Viral transcription is highly regulated, as demonstrated biochemically in viruses of the Reoviridae. mRNA transcription in these viruses is activated by external actions, for example, removal of their outer shell in multi-shelled reoviruses and binding of S-adenosyl-L-methionine (SAM) in the single-shelled cytoplasmic polyhedrosis virus (CPV). To reveal the mechanisms of transcriptional regulation of viruses within the Reoviridae family, we determined the cryoEM structures of six CPV/ligand complexes in the presence of magnesium ion: CPV+SAM (i.e., ‘S-CPV’), CPV+SAM+4 nucleoside triphosphates (NTPs) (i.e., transcribing, or ‘t-CPV’), CPV+SAM+GTP+ATP (i.e., ‘SGA-CPV’), CPV+SAM +GTP (i.e., ‘SG-CPV’), CPV+GTP (i.e., ‘G-CPV’), and CPV+ATP (i.e., ‘A-CPV’) at resolutions ranging from 2.9 to 3.1 Å. Like the atomic model of unliganded CPV, the atomic models of these liganded CPV all contain two conformers of the capsid shell proteins (CSP-A and CSP-B), two conformers of the large protrusion proteins (LPP-3 and LPP-5), and one conformer of TP in each asymmetrical unit. We discovered that the large sub-domain of guanylyltransferase (GTase) domain of CPV turret protein (TP) also has an ATP-binding site and is likely an ATPase that mediates the activation process of viral RNA transcription and capping.

Except for A-CPV, these atomic models also contain ligands revealed in our cryoEM maps. To test this hypothesis, we first obtained the 3D reconstructions of G-CPV and A-CPV at 2.9 Å and 3.1 Å resolutions, respectively. Our structures of G-CPV and A-CPV show that, in the absence of SAM, neither GTP nor ATP induced any conformational change.

> MWHYTSINNDTRVALDPKPNQIRTITKPNTVPQLGTDYLYTFNSQRRSHTLRLLGPFQYFNFSETDRGHPLFRLPLKYPSKAIPADELIDNLHSWMRSVHLLHVRSEDNTLRYNWMLGVYARSTNYTTPVGQLVVNAPAILNYSNPQDAFNSVFVALGIDYIDIPITNSNIFDDSSTPYNVRIWHAPTMTEVNHILALMRKSTLVSTHSSWHWNVLHTFHYRSESDMIDHFAAKILEDWRQKEKLDKGALVEADRVIQRLIPLSSSTYVQRLAAIGALYPNEFTENVLDLSRLSTALLQLSDTYYQHANDQLRRLYRRMYNDSRTLYMTQRHQELLLAQITADPNILLYPYTYIFTTIPTSMNYISNTGQGRIKHSLTVTGATEHDTVADIVLGQTGEDVITISMVEPMSIAVEDMYGYVLDTPTRDIWPADEQIEQKGDAVALYDTKTSRALGMFNNTVRIDDLLSPLLSLVYRTYIKGDTMTMTQGSLDHLTLCAAVDSDITFVGNRMIAPLPEGYIPKPMHRNNSTMKMLSLYVALKKLENFATNSYLMAPDTSIILLGAEREPAVNILRRFNRNVSNVRIIGMGDRAVEPNIRVRVPFPIDKNISADFIICDINSYEDQSFESMFSETISVVTTCASAATRALVKINHPSEYMINSVIERLSQLGGVFYHTALLKTASQNPYSYETYIYITPIAAAVRFPFYSNSAMINRYMTAVADDEMPIIPSIHTVIKGHSNTYSPGLFCGCVDVQSAPLALSQLKSYCSEATTWRVDSDDNLVNIIARIDPARIALEFRTRSNTSAYHEYQRYVPNGLGFKVRKTREFRYMHREVTFIHKLMMYALIREQISLTENMTQVVSIGGRNLADISVVPLNMKYVVIDPATRIETLTQEKKNIEVQSRPFQFDAANMDLENNSIYLFIAVIMNEPNGAATPARMQMDKIRNVATAMLTRTNCVAYISFYEAGIITRLDQSTAHKTIRVEEGRLKVANYVPVDTLVEADVTLMLRDIGITHEIIRPSTPELIDACSNYGIRLGSTGGAVLDVFNHYSPVIKLVRS;>MHSTNNNSNKRNNEEKHKQPEIDSSANNGEGTSGTRAQTVGDTATEAGVRNETEAGASTRRQTDGTGLSGTNAKIATASSARQADVEKPADVTFTIENVDDVGIMQQKKPPTVVQSRTDVFNEQFANEALHPTTKVIFNGLDVNTEVQPLSDDFKQISDPKGYLTYSVKYEDQFTKKDKLRASEADDRIVGPTVNLFKYGAAVVNIDLNRDFFDTATGIDLTKGIPLVQDLLVPIGVTAGAEQSAEYVSGLLMVLFKVMTDNRLVIVGETTTPMSNTLSTVVNNVLRTTYHNNVGVNPALLRDFTQVNWLNRDITNMLQQAGTKYGLGLTETRLDYVRLVKTIVGHALNIDHFAASVLNINLRALMEANVTADDRIKALQAHSMISTQFHGPNQGALRPELAFDHDHIIRCLMLAAANYPRLEGIIVQINTGYVASANVIRPVSEKRYFPENLEQNQSAARLVSAVKARASEADISSIHLAIAREVSPMFNVHELKKIAESFEDPSSIVVVLEFILFALFFPTEFNRIKGDIQNVLLLFFSRWYPVEYGIFVQRGATYTINAAGEFEFSGRNEKWDQALYLSEHFPALFSDVPLAGANTIIAIMRLFTPQGFLRTDDLAIAANFPRASRNPQTYIPYTNQRGTVTNEFASRFRTIVATLANVVNERAVQDDMQKATRSCTKQWLRHLETQFDNIAVAHTDHLSVVYATMSNFMLNFTNNFSGNHATFKPDQYVITSPEGSYKPIIERQGETVDGLTIIDTSIVWPILCQCTYPLVRQSGKGVDAVSIMEEIVYPDPSTTLSQSLSVAQVLSKLTLPDAFINMILSGGDSVVMRTYQTEADDDLDEGIRMTTYDQYLSHIRERLHITNVPDPIYITGASTPDQIAASVQATHVAVVLYQSGVINGPASTYLRENEVLVVMPDYYDVVSRFANANLQMNNNRYHESVLEIADIFDQADFIQTSDAVRQLRALMPTLSTSQIRHAIERIAQITDVDSTDYGKLTLRFLGTLTRSLKMQNAQIRRIRPDGTVLRYDDQIDIEAFRWSRYFLDELQLRRLSVGLRLITNPRIARRFNGVRIMYLTDDDPDPDFVPDVPEGYVAVQYAHRLFSSSLANKRNRVTYTHPPTGMAYPSPTGRPHVHMTINERAGMSKLVADNIIASVIKSNWVVDILDIEYTAEVMTPSEGYTQHVDAESIMTAPKGKLFHLQFMDGLLRPEPSAFDPPASGEDMRLIYPLQPISVARSMRAIVNHNEVDRPRGAVAPSSYEMDTGTLSRNGDLLYSPVANGQVGIPKLEVDHISFSNVVSMMTANIRTGDDMAVERVNPDDVRAINIRNA[2x];>[2x]MLQQPTGGYTTLEQFAFTIRNDGTNATPTQFLQLLSYEATENELVKKTIPTPETHLPSARNVPGNVYIEDAITQALFGISAQNVNAHGYFSRLSALALPNTSARLGLDGVIYNSETINIPFYDPAAVANFAATYAKLGNASTPRYRADMIDIYAHVGLELAGTDAERAAGVMPVKRAKFDSWEGSLISLSRDVVNWKILAFLIDLCSLEGEALRAFKTRNRDVFRMMLFIMSTAVAANVVNRKVTKRVDRVLEYIGVNSMRTAGRTATITYDLSRHEFAAKFLQLTFTRWNAASAMIRSMPDMHTPRTSITPAGENALVRHNRYMTENFKGLSPIALAQKKHEMMLHTHEIHSMDIDGSIKNMVERETVNKMNEIDAMNTAPWTEEFAEVEPTTVYERHQIGTDPEQTQLISQDAAVIVHQASSDVDENEYGNSVSELTIDTQSDSVL> GSAMGSFDRQLTEDQEVVLKQIWTHLFHLWQVPVDGTHIFPN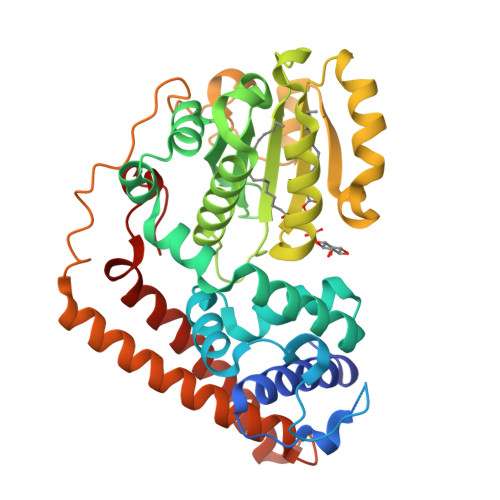NSLHSKKKSSWFSKLQDSSEAAEAAHLYEKGKIHKALANLDPQTTKKQFWHDIKNETPDATILKFIRARKWNADKTIAMLGHDLYWRKDTINKIINGGERAVYENNETGVIKNLELQKATIQGYDNDMRPVILVRPRLHHSSDQTEQELEKFSLLVIEQSKLFFKENYPASTTILFDLNGFSMSNMDYAPVKFLITCFEAHYPESLGHLLIHKAPWIFNPIWNIIKNWLDPVVASKIVFTKNIDELHKFIQPQYIPRYLGGENDNDLDHYTPPDGSLDVHLKDTETRAMIEKEREELVEQFLTVTAQWIEHQPLNDPAYIQLQEKRVQLSTALCENYSKLDPYIRSRSVYDYNGSLKV> MSLTSVVFLNPGNSTETFWVSYSQFMQAAARDLGLDLRILYAERDPQNTLQQARELFQGRDKPDYLMLVNEQYVAPQILRLSQGSGIKLFIVNSPLTLDQRELIGQSRQNYSDWIGSMVGDDEEAGYRMLKELLHKLGPVPAGHGIELLAFSGLKVTPAAQLRERGLRRALAEHPQVHLRQLVYGEWNRERAYRQAQQLLKRYPKTQLVWSANDEMALGAMQAAR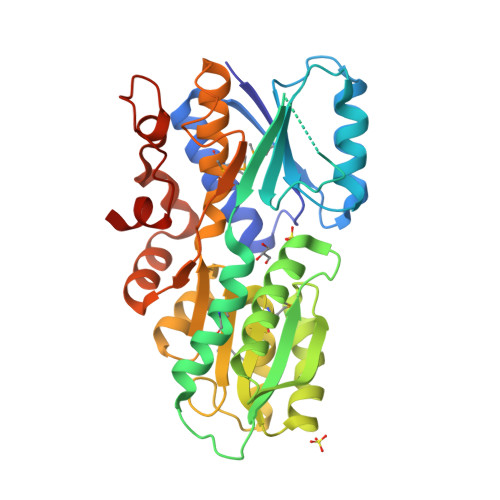ELGRKPGTDLLFSGVNSSPEALQALIDGKLSVLEAGHFTLGGWALVALHDDALGLDARRLGGPDWQLSLFQALTPAQARQLLRLGDQVGTRVDFRGLSAQGKPDSYRYPFGLQLLLREGHHHHHH>MATSPEGIWSNSGALTFEDPADDSEILFAGVRDVTITPAYEHAELYTIDSTFRDEVKRYEHNVNVEITYAKFSLEFAQEWLGGPGATATASQDDSDPMKFNLENVTPSASGGFERTTAVENVVFPELPLDSATYGEYEEYSLTGSGRSVTNLADTSGV[66x];>MVDATLSRGGTSVDIPLVEEGGEILLSSTFGKPEVNVRKSGGSLNPRVIDSWSGLQTFQLVGKLYDYSTSHQLADLVKTASTTPLELQIPQDAYPDTVTVAPAAGQASALTLEYPAGRKDLVDVSLSLTRVDPNSVRGVGDQQATTPTTTGTGPVEVTAGGTTVQLPSSGLSVERTVGRPNDAVRRVPRQADPRYEVKAKVTNDVFTFSFETLDNIPATLNALTDNVFREQLGRDGVTLDFNGLLGLGSVKAIPVGSSPFRQVHQAGRGWVTVPTLEFRRIYSNE[3x];>MPQLGDSKLGESQLGSPGTLKQGVEWTVVVDGEEQNNVWDVQVVDTANPFGDYAVFKMDDRGGQAFEAYPRGTRVEAYVSEGTEPLDNRFTGYVVERRENEQQGADVLEVEAYSFDQFLRRNTVTNDQTGNTISQALADIIQTDTPVRFNAANITVGDDQELTRSYQGDPVENALRDFAFKSTNEDFGVGDDLEFFFQPRETVHIDRGVDNTQWFRYDIPELGKEAINEVEVWFDDGEESVIVDDGTDKLDLQDSLGLPSPGTQRKELQRPLVTDISDAEDIGRKYLAFRNSTLSGTVTTYGLYDAEPGDTIDITIDPRGIDEEFVIAAIEYRWGVDETILTVVEKRGDVDDILSELSESVQRIEMQGANRDAPKNRITTTNAAAIVSVDVDAGGTSADADRFVNDGRNAVRDAWTGAGNPDIANIVVGDDNSGLSRTNTTLGNQTDSVSVTESLPSAKVVEYSATLTQSGVEEIGLETSTGTLLTRATFETPVDLSSDTVTVTLTVSNDDSVSRGVMTNDGQTAVRDVLADNSPTLPTDYGYGDDSTAVAETDTTLGNELANTSLEEILIQSASSVSAWNTILGTLASTYPLVVSSSGIRPAQTAWTTESDNLAQSGTALVTVGDYSNGEAEGLDSPGDTLELSFTPEHDIPGEEFALWCRIETDLGGTDPGPEITVTLDIDGDTYSWVPIGTNTALGLNWYDLANNTFGGSSTYPDTDIPEGSTVTLSIEATSSSVSGQGHAVDVMAPLDALTRVTGGSDATSAYTFDNNNGGSGGYLDGPELYPDQLILSLETATTRRNVSEARFTLTANDTSGNFYVELANDGSTFNRVNNATSGSVTFASPDTNVDTNISLNRYGSRSTATPQTGFNAQEIDNWELYADIDAVLPDDIGVTLSRAIIPPNTSGIVGQTVREAGLKSGSTLLTRHILAEFLLDTDQRLASSESTRFTSDN[3x];>[12x]MPKYNLRIGNRRVPIASTDTPLSEAIGKRLASSTPQTNVDSMGGGHSYQFNGQDLTFEDLRDIKDVRDSGGQVAQLMDYKALLNFGEGCEIHVEGDDETKQLVDGEPMTLSEWLEDAFPHLDLLVLDLGGDALWYPYAVGEIQETITGEFKEALPAEPWTLMPESDAQGKVQAWHQRTKTHGGYQTQTLPADDLWHIVINKASARDEVGISEVLRNKDEIQAFKQNEAAINQAIELHGFPQRHVKVGKEDGAPVRDNDLRRVRTIFDPRTTDANTAYFTGQDVDVETLEAHNFDYSAIHEMDMRNLTTALGLPLEAGNVGADGLGSGKPAELRFALLKLAIKANQRSFSVQFVERVMRPVVRDYSPFDHEADIRLEINDPLEDIGEVADLIQQVGDYMTNEQVAEKLDLPAPEDDEVADSYRSPADMEKDEAGVQDEPFGGMFAGRDMGNRCLGEGITDDELQHAPEWDRPLLEMYQGVTNPESDTSRTLVSFSSSGTPEFVLERIRESIMDGALFSEFDNIPSSRLMELRQTFADELGTDNFTLDSITDALMDFEADLTRDAAERIARTESSAVLNHAREISYEERGEGNELFYWTGADLGDSRQTEACAWLIRQTNPFSGGTPVPMNELRDMVDEAPSHDDSMDNNLARPDSWVVHPNERSSFVKAPPNWEQL;>[12x]MPDPSIDEVSKSDWDALTTQEQDDIISQVENLSSTGWVNTSRERKAEAIRSAIAERDTLYSGNMSRLPTLDGDAEYFTLYLSAHKIQLFEGGEAQSESGEGGSVSYSTGGGGEKDLQKTRYGRMALEYVWEDNSIAALRTY;>[6x]MATTSASHHVQAIIDLLEAAPDADWTPTQTPTVKRYWDDAQSERGPGADMPAILYVWSPTTSSLDRFSMDGDVFDQNDSIEVQAWSFDETEVEQLQGDIVQILSEYLDDNEVQTPYSDVAPTGTNDFREQTPARTTGHYIMSVEVETRGLSETAKNA;>MVAIRSEGVSETQQNLEGVENAMEDTADSAGDSAAELETFSKRFKGAMGAAVSALAIGTAGLLSQVPVVGEAMGGLGAIIDALTMKIDEDARPAVGSFTDDLYEVAEATYEADSSLEAFQTALDGVNTAIDDVAVSTLQTEIEELTGITIPKNWLDFGWDIMTLDARQTMDNIETIINEFPEDFGTMLKSIDPRAKKGWDILTKSADMFINDLTSRIDSGVNDVRGFFTGLASDLNEWGGNVASDAREWGTNLIDKFTGGIRSKISGLRNWLSELRNIGAEVGIDVPTIGGGGDGGGGGGNSSRQPFAGGFFGGGNATIDGRQISESTGRYRSDPSRRRGI[6x]

Here, we present the near-atomic resolution structure of Haloferax tailed virus 1 (HFTV1), an archaeal virus thriving in extreme salinity. Through single-particle analysis, we obtained near-atomic resolution maps of DNA-filled and empty virions, enabling us to assemble full atomic models of the virus pre- and post-DNA release, including all structural protein components. The full atomic structure revealed that the virus has a length of 1350 Å and an icosahedral head with a diameter of ~600 Å. The tail has a length of 560 Å and terminates into a baseplate with three radiating TFs of ~190 Å in length.

(A) Full structure of the tail consisting of a dodecameric head-tail connector (HTC), a hexameric tail completion protein (TCP), 11 tail tube (TTP) hexamers, a trimeric baseplate-tail connector (BTC), a trimeric baseplate hub (BPH), and three trimeric tail fibers (TFs). The tail region begins with dodecameric gp26 [head-tail connector (HTC)], which interacts with the PP to maintain a conduit through which DNA can pass. This is followed by hexameric gp29 [tail completion protein (TCP)], and subsequently, 11 copies of hexameric gp35 [tail tube protein (TTP)] making up the bulk of the tail. Each hexameric segment of the tail is rotationally offset from the next by 23.6°. The tail forms a hollow tunnel of 36 Å in diameter. In the DNA-filled virus, this tunnel houses gp40 (TMP), a hexameric coiled-coil structure with alternating C-terminal conformations. The TMP extends from the central channel of the first TTP near the portal to a cavity in gp44 [baseplate hub (BPH)]. The coiled-coil region of the TMP precisely aligns with the 11 tail tube rings, confirming that its length dictates tail tube length. In addition, we observe two densities between the DNA and the TMP, located within the TCP and HTC proteins. Because of its location between the TMP and DNA, we name this protein the TMP-DNA spacer (TDS). The TMP and dsDNA are separated by a spacer (TDS), and the dsDNA traverses through the portal into the capsid.>[2x]GPMVSLAQVRGALCGALLGDCMGAEFEGSDAVELPDVLEFVRLLEKEKKAGTLFYTDDTAMTRAVIQSLIAKPDFDEVDMAKRFAEEYKKEPTRGYGAGVVQVFKKLLSPKYSDVFQPAREQFDGKGSYGNGGAMRVASIALAYPNIQDVIKFARRSAQLTHASPLGYNGAILQALAVHFALQGELKRDTFLEQLIGEMERIEGGEMSASDAGEHDRPNEVKLPFCSRLKKIKEFLASSNV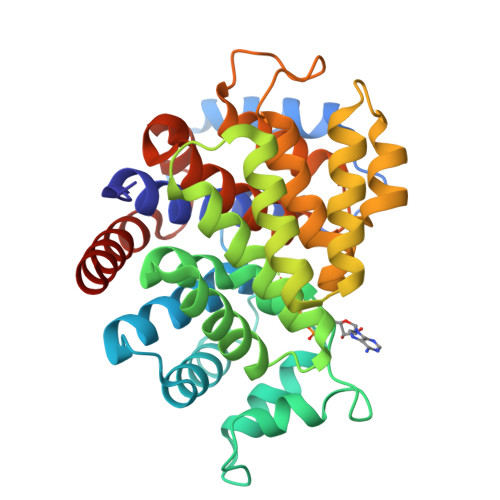PKADIVDELGHGIAALESVPTAIYSFLHCMESDPDIPDLYNNLQRTIIYSISLGGDTDTIATMAGAIAGAYYGMDQVTPSWKRSCEAIVETEESAVKLYELYCKQLKTP>[2x]MKMASNDAAPSNDGATGLVPEINNETLPLEPVAGAAIAAPVTGQNNIIDPWIRTNFVQAPNGEFTVSPRNSPGEILLNLELGPDLNPYLAHLSRMYNGYAGGVEVQVLLAGNAFTAGKILFAAVPPNFPVEFLSPAQITMLPHLIVDVRTLEPIMIPLPDVRNTFFHYNNQPANRMRLVAMLYTPLRSNGSGDDVFTVSCRVLTRPTPDFEFTYLVPPSVESKTKPFSLPILTISELTNSRFPAPIDSLFTAQNNNLNVQCQNGRCTLDGELQGTTQLLPSGICAFRGRLTADVDGSHDDRWHMQLTNLNGTPFDPTEDVPAPLGTPDFTGLLFGVASQRNVGSNPNTTRAHEAVVSTTSSQFVPKLGSVNFGSTSTDFQLQQPTKFTPVGIKIESGHEFDQWALPRYSGHLTLNMNLAPPIAP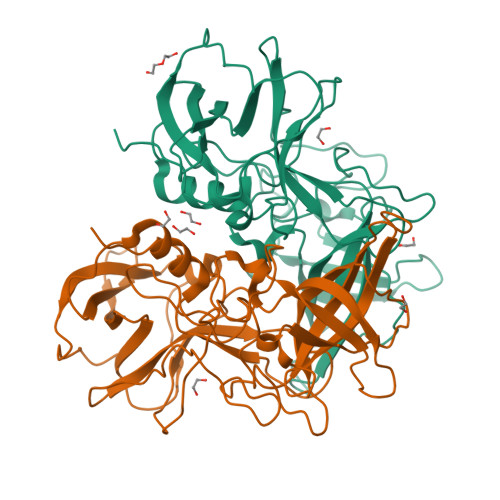NFPGEQLLFFRSNVPCAGGVSDGVIDCLLPQEWIQHFYQESAPSQSDVALIRYVNPDTGRTLFEAKLHRTGYITVAHSGDYPLVVPSNGYFRFDSWVNQFYSLAPMGTGNGRRRVQ> GRNVTVE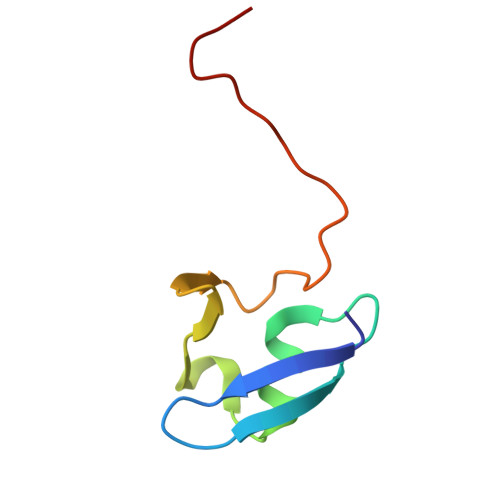VVGEETSEVAVDDDGTYADLVRAVDLSPHEVTVLVDGRPVPEDQSVEVDRVKVLRLIKGG>[10x]MSKIERISAFLNDKEVDMTFITNPTTLNYLTGLAIDPHERIAGLMIFRDSTPMLFTPALEVEKAKEHTSGLDIFGYEDSQNPWEVVKNHVKSDVKSIAVEFSDIPLAKTEGL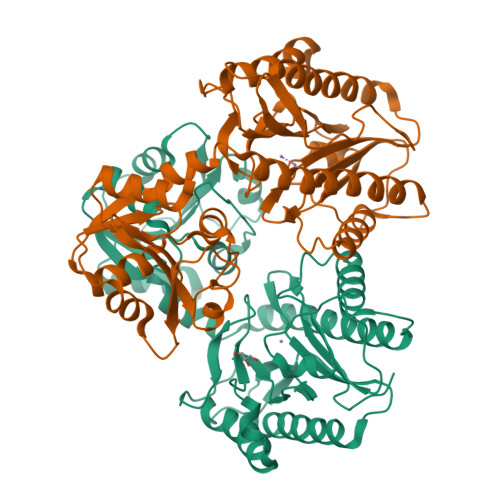KAQFGDINFVNLTPLIERMRLIKSADEIEKMKVAGDFADKCFEIGFATAAERNGVTESDIVAKIEYEMKRMGVPQMSFDTLVLSGARAANPHGAPENVEIQENKLLLFDLGVMSGGYASDATRTIAIGQPNDFDAEIHKIVKEAQQAAMDFIKPGVTAHEVDAVARDLITKAGYGEYFNHSLGHGIGMDVHEYPSIVAGNDLVIQEGMCFSNEPGIYIPGKVGVRIEDCLYVTENGCESFTHTDHDLLIF> MGLEQLEAQTNFTKRELQVLYRGFKNECPSGVVNEDTFKQIYAQFFPHGDASTYAHYLFNAFDTTQTGSVKFEDFVTALSILLRGTVHEKLRWTFNLYDINKDGY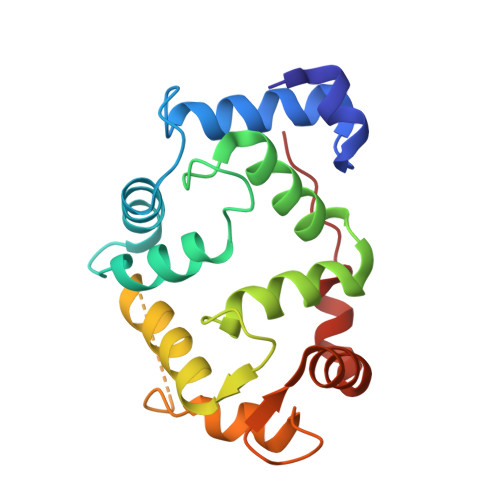INKEEMMDIVKAIYDMMGKYTYPVLKEDTPRQHVDVFFQKMDKNKDGIVTLDEFLESCQEDDNIMRSLQLFQNVM> MGSSHHHHHHSSGRENLYFQGMIKEMIEDFISKGGLIFTHSGRYTNTNNSCFIFNKNDIGVDTKVDMYTPKSAGIKNEEGENLWQVLNKANMFYRIYSGELGEELQYLLKSCCTAKEDVTTLPQIYFKNGEGYDILVPIGNAHNLISGT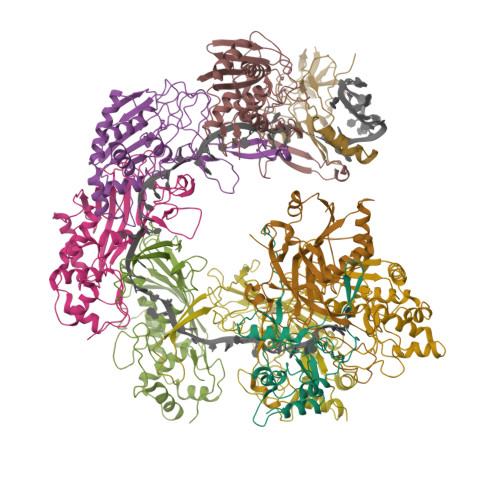EYLWEHKYYNTFTQKLGGSNPQNCTHACNKMRGGFKQFNCTPPQVEDNYNA;> MGSSHHHHHHSSGRENLYFQGMRKFIIVKNVKVDGINAKSSDITVGMPPATTFCGLGETMSIKTGIVVKAVSYGSVKFEVRGSRFNTSVTKFAWQDRGNGGKANNNSPIQPKPLADGVFTLCFEVEWEDCAEVLVDKVTNFINTARIAGGTIASFNKPFVKVAKDAEELASVKNAMMPCYVVVDCGVEVNIFEDAVNRKLQPMVNGYKKLEKIVDNKHMRDKFTPAYLATPTYTMIGYKMVSNVDNFDQALWQYGENTKVKTIGGIYND;>[6x]MGSSHHHHHHSSGRENLYFQGMTKLKAPAVLAYSRKINPTNALMFAVNWSDRDNTTAVMVGTKTVAGTQSVRGNPNDADKGNIQTVNFANLPHNKNTLLVKYNVKFVGDVFKAELGGGEYSNTLQTALENTDFGTLAYRYVYNIAAGRTLWRNRVGAESIETVITVNDQTFTFSDLLVNEFDEDVDVAEIADMVAGVLSGEGFVTLKVEHYMLLGEGSEVFPSQEFVENSKLSKQLFDLNGQAAMHDQKIGNAIRTIDTWYEDATTPIAVEPYGSVVRNGVAYRAGNKTDLFTLMDGAVNGKSLTEEDQMFVTANLIRGGVFGGGKD;> MGSSHHHHHHSSGRENLYFQGMYNTISITVVDADDVGVNFVVSKVLSTLHNKGIFNGEVGVTFPRMDKNVGDIITLFSKTGVDRKVLTSTLNTLTDFIHIGKPKEADKVKTYRKVDTKSKGKLIRRCIKRKGVSAETAESLYGNYKGEKCKLPYIVVNSKSTGQRFSMFLEECENSEKFNSYGLCIVSC N-hydroxy-2-{4-[3-(4-{[(2R)-2-hydroxy-3,3-dimethylbutyl]oxy}-3-methylphenyl)pentan-3-yl]-2-methylphenoxy}acetamide | C27 H39 N O5 | 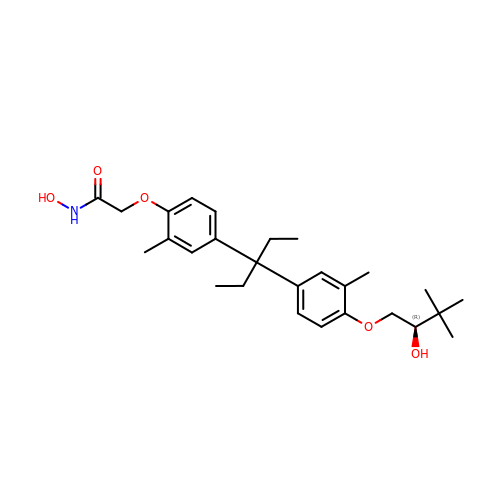HLEDBIQBAUIWNJ-DEOSSOPVSA-N>GUAUACAC[4x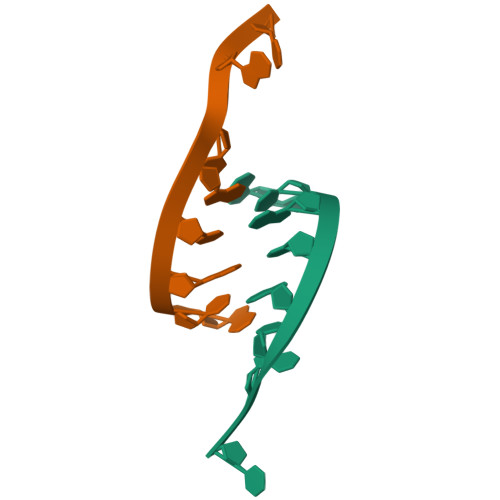]>GETKKMICLVDGEHYFPVVKDSIEILDDLEHIDVVAVVFIGGTEKLQIEDPKEYSEKLGKPVFFGPDPKKIPYDVIKKCVKKYNADIVMDLSDEPVVDYTKRFRIASIVLKEGAVYQGADFKFEPLTEYDVLEKPSIKIIGTGKRIGKTAVSAYAARVIHKHKYNPCVVAMGRGGPREPEIVEGNKIEITAEYLLEQADKGVHAASDHWEDALMSRILTVGCRRCGGGMLGDTFITNVKRGAEIANKLDSDFVIMEGSGAAIPPVKTNRQIVTVGANQPMININNFFGPFRIGLADLVIITMCEEPMATTEKIKKVEKFIKEINPSANVIPTVFRPKPVGNVEGKKVLFATTAPKVVVGKLVNYLESKYGCDVVGVTPHLSNRPLLRRDLKKYINKADLMLTELKAAAVDVATRVAIEAGLDVVYCDNIPVVIDESYGNIDDAIIEVVEMAIDDFKNNR[4x]

The enzyme cyclic di-phosphoglycerate synthetase that is involved in the production of the osmolyte cyclic 2,3-diphosphoglycerate has been studied both biochemically and structurally. The reaction involves the transfer of the γ-phosphate group from ATP to the substrate 2,3 -diphosphoglycerate and the subsequent SN2 attack to form a phosphoanhydride. The unique structure of cDPGS is made up of an N-terminal domain which is crucial for the stabilization of the active dimeric structure and the ligand interactions, and a C-terminal domain that contains a P-loop kinase fold as part of its structure. Since the cDPGS reaction is exergonic at cellular concentrations, cDPG accumulation is favored thermodynamically until this reaction reaches equilibrium. cDPG appears to play a role in the thermoprotection of proteins, and increased thermostability has been demonstrated for several model enzymes in its presence.

To elucidate the substrate binding residues of cDPGS, the structure of the 2,3 DPG, ADP/Mg2+ bound enzyme complex was solved by molecular replacement to a resolution of 2.2 Å resolution, resulting in Rwork and Rfree values of 21.5 and 25.6%, respectively. The 2,3 DPG binding site is located between the C-terminal domain of the one protomer and the N-terminal domain of the other protomer of the dimer. The ADP and Mg2+ are clearly resolved and reside in the pocket formed within the C-terminal domain. The 2,3 DPG is clearly resolved in only three of the four protomers making up the asymmetric unit of the crystal. A phosphate molecule has been modeled in the active site of the 4th protomer. The Walker A/P-loop surrounds the pyrophosphate moiety of the ADP while coordinating with the Mg2+ atom. A superposition of the apo- and ADP/Mg2+ bound forms of cDPGS reveals a large movement of several α-helices that close around the nucleotide, which highlight the significant conformational changes that accompany ligand binding. The helices α5, α8, α9 and α14 show a motion of up to 8.5, 7.0, 6.7, and 2.6 Å, respectively. A closer look at the active site revealed that the closure is triggered by the binding of the substrate and ADP which brings the Walker A/P-loop close enough to contribute to the stabilization of 2,3 DPG. Residues K145 and R146 move closer to the substrate to form multiple hydrogen bonds with it.> SDKKSLMPLVGIPGEIKNRLNILDFVKNDKFFTLYVRALQVLQARDQSDYSSFFQLGGIHGLPYTEWAKAQPQLHLYKANYCTHGTVLFPTWHRAYESTWEQTLWEAAGTVAQRFTTSDQAEWIQAAKDLRQPFWDWGYWPNDPDFIGLPDQVIRDKQVEITDYNGTKIEVENPILHYKFHPIEPTFEGDFAQWQTTMRYPDVQKQENIEGMIAGIKAAAPGFREWTFNMLTKNYTWELFSNHGAVVGAHANSLEMVHNTVHFLIGRDPTLDPLVPGHMGSVPHAAFDPIFWMHHCN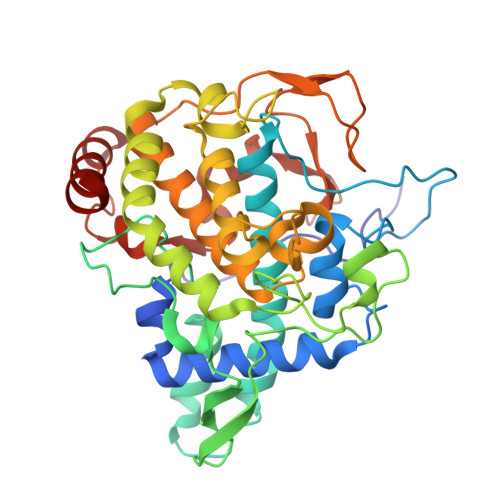VDRLLALWQTMNYDVYVSEGMNREATMGLIPGQVLTEDSPLEPFYTKNQDPWQSDDLEDWETLGFSYPDFDPVKGKSKEEKSVYINDWVHKHYG> ATITQDTPINQIFTDTALAEKMKTVLGKTNVTDTVSQTDLDQVTTLQADRLGIKSIDGVEYLNNLTQINFSNNQLTDITPLKNLTKLVDILMNNNQIADIT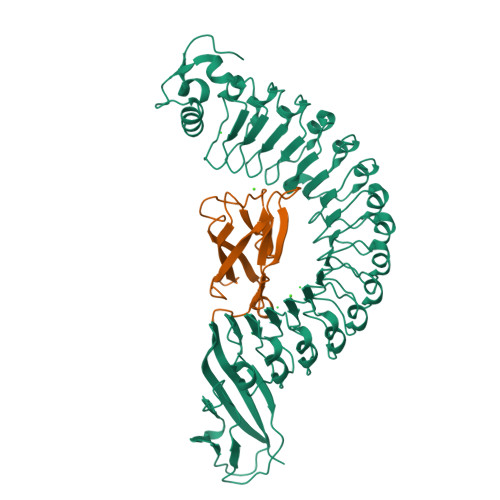PLANLTNLTGLTLFNNQITDIDPLKNLTNLNRLELSSNTISDISALSGLTSLQQLNFGNQVTDLKPLANLTTLERLDISSNKVSDISVLAKLTNLESLIATNNQISDITPLGILTNLDELSLNGNQLKDIGTLASLTNLTDLDLANNQISNLAPLSGLTKLTELKLGANQISNISPLAGLTALTNLELNENQLEDISPISNLKNLTYLTLYFNNISDISPVSSLTKLQRLFFYNNKVSDVSSLANLTNINWLSAGHNQISDLTPLANLTRITQLGLNDQAWTNAPVNYKANVSIPNTVKNVTGALIAPATISDGGSYTEPDITWNLPSYTNEVSYTFSQPVTIGKGTTTFSGTVTQPLKA;> GPLGSWVIPPISCPENEKGPFPKNLVQIKSNKDKEGKVFYSITGQGADTPPVGVFIIERETGWLKVTEPLDRERIATYTLFSHAVSSNGNAVEDPMEILITVTDQ> SNAMDVEKDVLDVYIKNLENQIGNKRYFLKQAQGAIDEITKRSLDTEGKPVNSEVFTELLRKPMFFSERADPIGFSLTSNFLSLRAQSSSEWLSL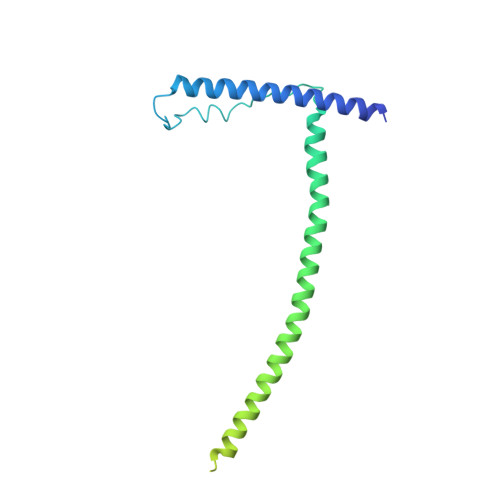MNDQSVDQKAMLLLQNNINSDLKELLRKLQHQMTIMDSKKQDHAHIRTRKARNKELWDSLADFLKGYLVPNLDDNDESIDSLTNEVMLLMKRLIEHDLNLTLNDFSSKTIPIYRLLLRANIITVIEGSTNPGTKYIKLIDFNETSLT> MTTEQRRSLQAFQDYIRKTLDP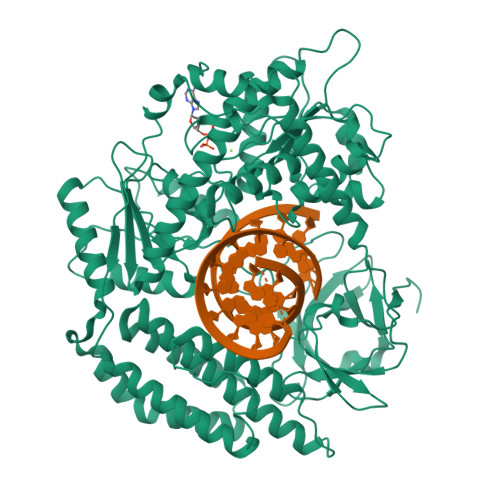TYILSYMAPWFREEEVQYIQAEKNNKGPMEAATLFLKFLLELQEEGWFRGFLDALDHAGYSGLYEAIESWDFKKIEKLEEYRLLLKRLQPEFKTRIIPTDIISDLSECLINQECEEILQICSTKGMMAGAEKLVECLLRSDKENWPKTLKLALEKERNKFSELWIVEKGIKDVETEDLEDKMETSDIQIFYQEDPECQNLSENSCPPSEVSDTNLYSPFKPRNYQLELALPAMKGKNTIICAPTGCGKTFVSLLICEHHLKKFPQGQKGKVVFFANQIPVYEQQKSVFSKYFERHGYRVTGISGATAENVPVEQIVENNDIIILTPQILVNNLKKGTIPSLSIFTLMIFDECHNTSKQHPYNMIMFNYLDQKLGGSSGPLPQVIGLTASVGVGDAKNTDEALDYICKLCASLDASVIATVKHNLEELEQVVYKPQKFFRKVESRISDKFKYIIAQLMRDTESLAKRICKDLENLSQIQNREFGTQKYEQWIVTVQKACMVFQMPDKDEESRICKALFLYTSHLRKYNDALIISEHARMKDALDYLKDFFSNVRAAGFDEIEQDLTQRFEEKLQELESVSRDPSNENPKLEDLCFILQEEYHLNPETITILFVKTRALVDALKNWIEGNPKLSFLKPGILTGRGKTNQNTGMTLPAQKCILDAFKASGDHNILIATSVADEGIDIAQCNLVILYEYVGNVIKMIQTRGRGRARGSKCFLLTSNAGVIEKEQINMYKEKMMNDSILRLQTWDEAVFREKILHIQTHEKFIRDSQEKPKPVPDKENKKLLCRKCKALACYTADVRVIEECHYTVLGDAFKECFVSRPHPKPKQFSSFEKRAKIFCARQNCSHDWGIHVKYKTFEIPVIKIESFVVEDIATGVQTLYSKWKDFHFEKIPFDPAEMSK> ASGADIVLFSGSKHVEFTDWGGT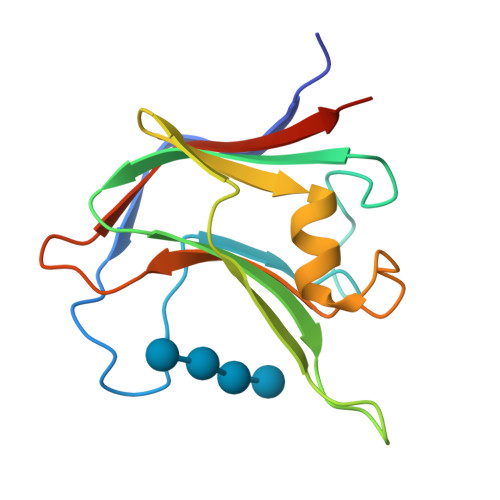DWPSAYELQPPYQTMPFDLNKNFEIKVDYSGADIVLIFARWEHGSKPQIWAQISPYYVVDGTAVFTKEQIAKAYGSDDFSDLDYIGVKPLPSADGMTVTKIVASYTSGSSDD>[4x]MKTELTLNVLQTMNAQEYEDIRA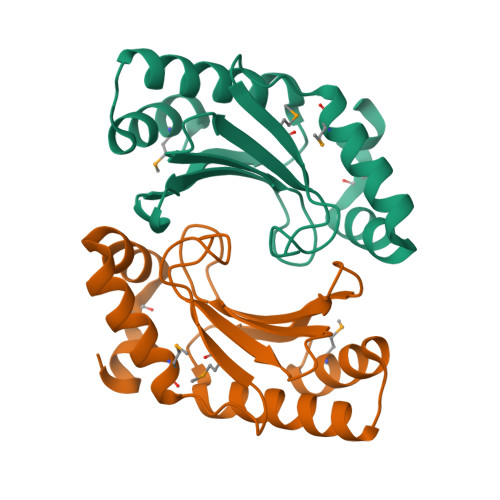AGSDERRELTHAVMRELDAPDNWTMNGEYGSEFGGFFPVQVRFTPAHERFHLALCSPGDVSQVWVLVLVNAGGEPFAVVQVQRRFASEAVSHSLALAASLDTQGYSVNDIIHILMAEGGQV>[4x]TPTSNDACLSIVHSLMCHRQGGESET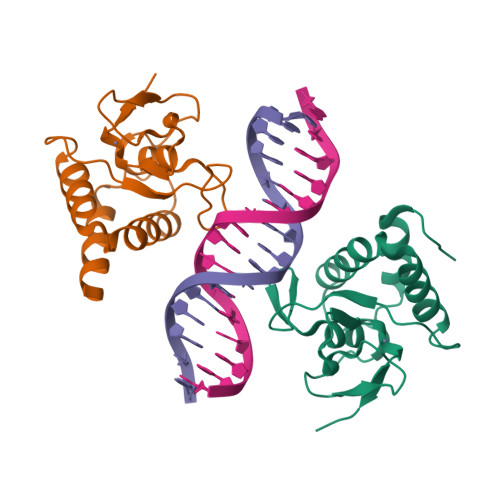FAKRAIESLVKKLKEKKDELDSLITAITTNGAHPSKCVTIQRTLDGRLQVAGRKGFPHVIYARLWRWPDLHKNELKHVKYCQYAFDLKCDSVCVNPYHYERVVSPG>MSIEKLKAALPEYAKDIKLNLSSITRSSVLDQEQLWGTLLASAAATRNPQVLADIG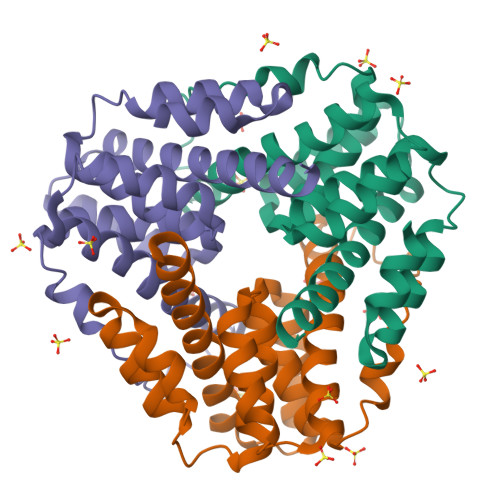AEATDHLSAAARHAALGAAAIMGMNNVFYRGRGFLEGRYDDLRPGLRMNIIANPGIPKANFELWSFAVSAINGCSHCLVAHEHTLRTVGVDREAIFEALKAAAIVSGVAQALATIEALSPS[3x]> MSSPDFSAGRELRTQGARIAGVVSCVPSKQVDNDYFVERFDASAVRDVVKMIGVNRRRWADAQTSAGDLCRKAGEKLLAGLGWQADSIDALIFVSQTPNYRLPATAFVLQAELDLPASCLALDINLGCSGYPQALWLGMNLIQTGAAKRVLLAVGDTISKMIDPTDRSTSLLFGDAGTMTALETSNGDAAAHFIIGADGKGARNLIVPSGGFKPYDAAADERMAGKSPECLFMDGGE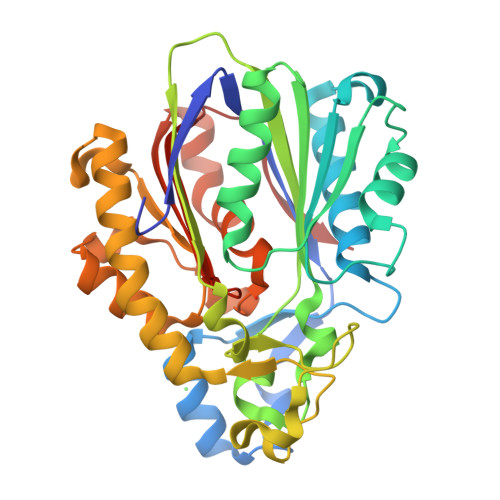IFNFTLNAVPKLVSRTLDIAGRDKDSYDAFLFHQANLFMLKHLAKKAGLPAERVPVNIGEYGNTSCASIPLLITTELKDRLKEETLQLGMFGFGVGYSWASAALAVGPLNIVDTIET> MKLPTNLAYERSIDPSDVCFFVVWPDDRKTPLTYNSRTLLGQMEAASLAYDVSGQPIKSATAEALAQGNPHQVDFCHVPYGASHIECSFSVSFSSELRQPYKCNSSKVKQTLVQLVELYETKIGWTELATRYLMNICNGKWLWKNTRKAYCWNIVLTPWPWNGEKVGFEDIRTNYT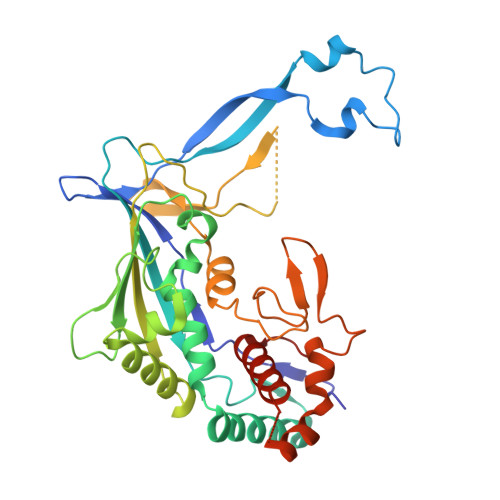SRQDFKNNKNWSAIVEMIKTAFSSTDGLAIFEVRATLHLPTNAMVRPSQVFTEKESGSKSKSKTQNSRVFQSTTIDGERSPILGAFKTGAAIATIDDWYPEATEPLRVGRFGVHREDVTCYRHPSTGKDFFSILQQAEHYIEVLSANKTPAQETINDMHFLMANLIKGGMFQHKGD>[12x]MGSDKIHHHHHHMAFFDLPLEELKKYRPERYEEKDFDEFWEETLAESEKFPLDPVFERMESHLKTVEAYDVTFSG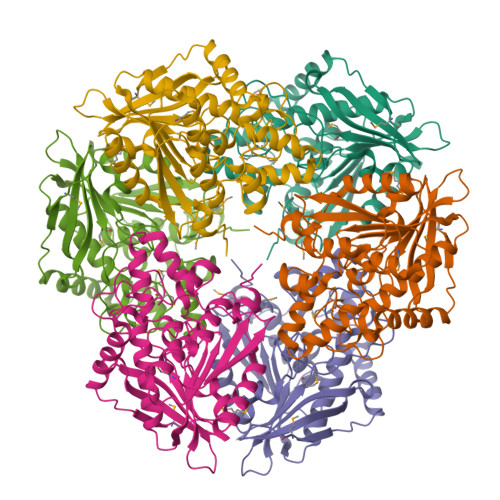YRGQRIKGWLLVPKLEEEKLPCVVQYIGYNGGRGFPHDWLFWPSMGYICFVMDTRGQGSGWLKGDTPDYPEGPVDPQYPGFMTRGILDPRTYYYRRVFTDAVRAVEAAASFPQVDQERIVIAGGSQGGGIALAVSALSKKAKALLCDVPFLCHFRRAVQLVDTHPYAEITNFLKTHRDKEEIVFRTLSYFDGVNFAARAKIPALFSVGLMDNICPPSTVFAAYNYYAGPKEIRIYPYNNHEGGGSFQAVEQVKFLKKLFEKG> TLPFRIGHGFDLHRLEPGYPLIIGGIVIPHDRGCEAHSDGDVLLHCVVDAILGALGLPDIGQIFPDSDPKWKGAASSVFIKEAVRLMDEAGYEIGNLDATLILQRPKISPHKETIRSNLSKLLGADPSVVNLK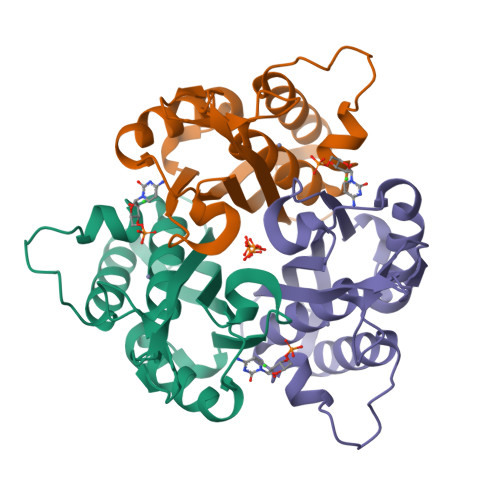AKTHEKVDSLGENRSIAAHTVILLMKK>[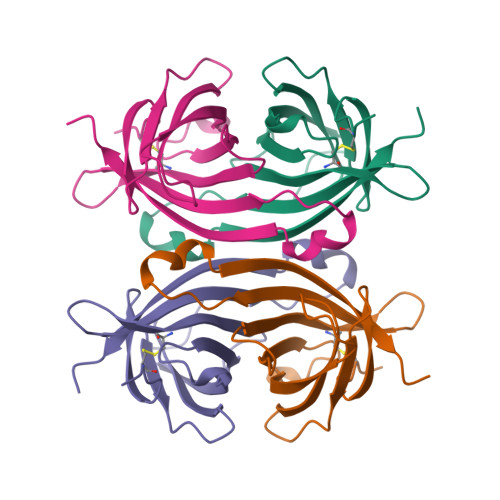2x]RKCSLTGKWTNDLGSNMTIGAVNSRGEFTGTYITAVTATSNEIKESPLHGTENTINKRTQPTFGFTVNWKFSESTTVFTGQCFIDRNGKEVLKTMWLLRSSVNDIGDDWKATRVGINIFTRLRTQKE>[2x]MAHHHHHHMSEATDTPPVDENKLIAERREKLKALRGQGIAYPNDFRREDFAGRLQEEFADAETWTAEALEGNGRQVKMAGRLMAKRIMGKASFAQIQDESGRIQLFLQGAVLGDAYTAFKGWDVGDIIAVEGGLTRTKTGELSVKAESIRLLTKSLRPLPDKWHGLADVEQRYRQRYVDLIVTPESRAVFIKRSKIIRAMRAWLDNRDFLEVETPMMHYIPGGAAAKPFTTHHNALDLDLYLRVAPELYLKRLTVGGLERVYEINRNFRNEGVSTRHNPEFTMMELYEAYATYNEIMDLTEGVIRDVAKAVNGGTEVEWDGAKIDLGPAFRRWRMDEAVRHHNPEISAADCTDRDALLRHCERLKIRVKPSYGWGKLLLEIFEATVEHTLIQPTFITDHPVEVSPLARANDNDPGYTDRFELFVNGKELANGFSELNDPEDQAQRFQAQVAAKE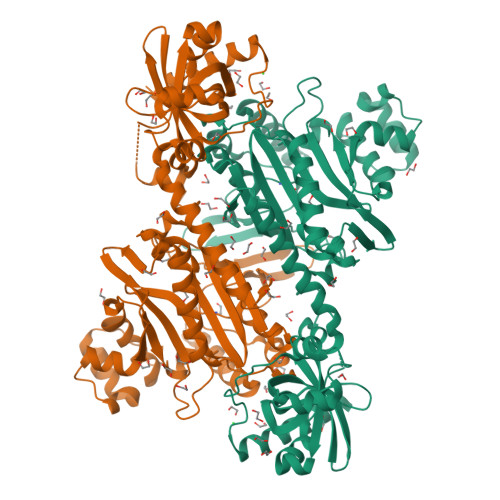GGDDEAMHYDADYIRALEYGMAPTGGLGIGVDRLVMLLTGSSSIRDVLLFPYMRPEQ>TETTSFSITKFGPDQQNLIFQGDGYTTKERLTLTKAVRNTVGRALYSSPIHIWDSKTGNVANFVTSFTFVIDAPNSYNVADGFTFFIAPVDTKPQTGGGYLGVFNSKDYDKTSQTVAVEFDTFYNTAWDPSNGDRHIGIDVNSIKSINTKSWALQNGKEANVVIAFNAATNVLTV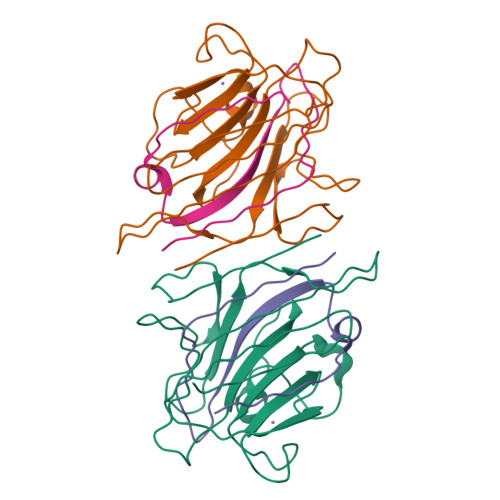SLTYPN[2x];>[2x]ETSYTLNEVVPLKEFVPEWVRIGFSATTGAEFAAHEVLSWYFHSELAGTSSS> GPHMGRAESGPEKPHLNLWLEAPDLLLAEVDLPKLDG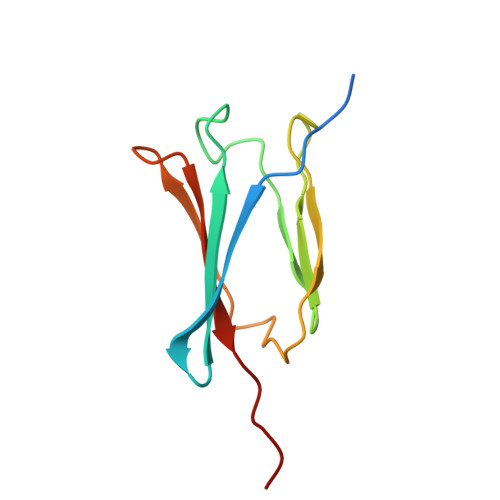ALGLSLEIGENRLVMGGPQQLYHLDAYIPLQINSHESKAAFHRKRKQLMVAMPLLPVPS dimethyl 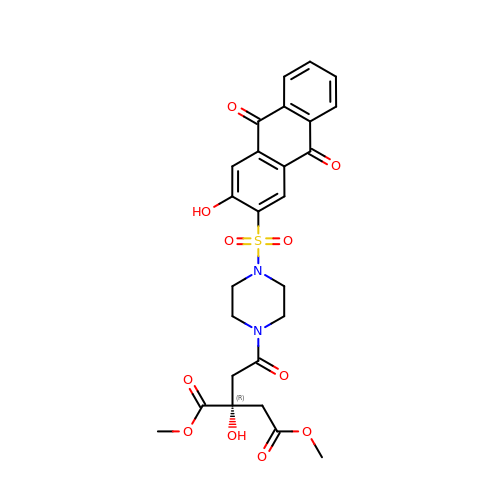(2R)-2-hydroxy-2-{2-[4-(3-hydroxy-9,10-dioxo-9,10-dihydroanthracene-2-sulfonyl)piperazin-1-yl]-2-oxoethyl}butanedioate | C26 H26 N2 O11 S | RCVSIAGVCLZIRH-AREMUKBSSA-N>MVEHDKSGSKRQELRSNMRNLITLNKGKFKPTASTAEGDEDDLSFTLLDSVFDTLSDSITCVLGSTDIGAIEVQQFMKDGSRNVLASFNIQTFDDKLLSFVHFADINQLVFVFEQGDIITATYDPVSLDPAETLIEIMGTIDNGIAAAQWSYDEETLAMVTKDRNVVVLSKLFEPISEYHLEVDDLKISKHVTVGWGKKETQFRGKGARAMEREALASLKASGLVGNQLRDPTMPYMVDTGDVTALDSHEITISWRGDCDYFAVSSVEEVPDEDDETKSIKRRAFRVFSREGQLDSASEPVTGMEHQLSWKPQGSLIASIQRKTDLGEEDSVDVIFFERNGLRHGEFDTRLPLDEKVESVCWNSNSEALAVVLANRIQLWTSKNYHWYLKQELYASDISYVKWHPEKDFTLMFSDAGFINIVDFAYKMAQGPTLEPFDNGTSLVVDGRTVNITPLALANVPPPMYYRDFETPGNVLDVACSFSNEIYAAINKDVLIFAAVPSIEEMKKGKHPSIVCEFPKSEFTSEVDSLRQVAFINDSIVGVLLDTDNLSRIALLDIQDITQPTLITIVEVYDKIVLLRSDFDYNHLVYETRDGTVCQLDAEGQLMEITKFPQLVRDFRVKRVHNTSAEDDDNWSAESSELVAFGITNNGKLFANQVLLASAVTSLEITDSFLLFTTAQHNLQFVHLNSTDFKPLPLVEEGVEDERVRAIERGSILVSVIPSKSSVVLQATRGNLETIYPRIMVLAEVRKNIMAKRYKEAFIVCRTHRINLDILHDYAPELFIENLEVFINQIGRVDYLNLFISCLSEDDVTKTKYKETLYSGISKSFGMEPAPLTEMQIYMKKKMFDPKTSKVNKICDAVLNVLLSNPEYKKKYLQTIITAYASQNPQNLSAALKLISELENSEEKDSCVTYLCFLQDVNVVYKSALSLYDVSLALLVAQKSQMDPREYLPFLQELQDNEPLRRKFLIDDYLGNYEKALEHLSEIDKDGNVSEEVIDYVESHDLYKHGLALYRYDSEKQNVIYNIYAKHLSSNQMYTDAAVAYEMLGKLKEAMGAYQSAKRWREAMSIAVQKFPEEVESVAEELISSLTFEHRYVDAADIQLEYLDNVKEAVALYCKAYRYDIASLVAIKAKKDELLEEVVDPGLGEGFGIIAELLADCKGQINSQLRRLRELRAKKEENPYAFYGQETEQADDVSVAPSETSTQESFFTRYTGKTGGTAKTGASRRTAKNKRREERKRARGKKGTIYEEEYLVQSVGRLIERLNQTKPDAVRVVEGLCRRNMREQAHQIQKNFVEVLDLLKANVKEIYSISEKDRERVNENGEVYYIPEIPVPEIHDFPKSHIVDF[2x];> MVECITPEAIFIGANKQTQVSDIHKVKKIVAFGAGKTIALWDPIEPNNKGVYATLKGHEAEVTCVRFVPDSDFMVSASEDHHVKIWKFTDYSHLQCIQTIQHYSKTIVALSALPSLISVGCADGTISIWRQNIQNDEFGLAHEFTIKKGFFYPLCLSLSKVEEKKYLLAIGGTNVNVFIASFILSDSGIEKCRVVAELEGHEDWVKSLAFRHQETPGDYLLCSGSQDRYIRLWRIRINDLIDDSEEDSKKLTLLSNKQYKFQIDDELRVGINFEALIMGHDDWISSLQWHESRLQLLAATADTSLMVWEPDETSGIWVCSLRLGEMSSKGASTATGSSGGFWSCLWFTHERMDFFLTNGKTGSWRMWATKDNIICDQRLGISGATKDVTDIAWSPSGEYLLATSLDQTTRLFAPWIYDASGRKREIATWHEFSRPQIHGYDMICVETVTDTRFVSGGDEKILRSFDLPKGVAGMLQKFVGIQFEEKSEMPDSATVPVLGLSNKAGEDDANEDDEEEEGGNKETPDITDPLSLLECPPMEDQLQRHLLWPEVEKLYGHGFEITCLDISPDQKLIASACRSNNVQNAVIRIFSTENWLEIKPALPFHSLTITRLKFSKDGKFLLSVCRDRKWALWERNMEDNTFELRFKNEKPHTRIIWDADWAPLEFGNVFVTASRDKTVKVWRHQKEPADDYVLEASIKHTKAVTAISIHDSMIREKILISVGLENGEIYLYSYTLGKFELITQLNEDITPADKITRLRWSHLKRNGKLFLGVGSSDLSTRIYSLAYE;> MARHGKGPKTNKKKLAPEKERFIQCCADITLELTDSLTSGTTREINLNGLITKYSKKYKLKQQPRLTDIINSIPDQYKKYLLPKLKAKPVRTASGIAVVAVMCKPHRCPHIAYTGNICVYCPGGPDSDFEYSTQSYTGYEPTSMRAIRARYDPYEQARGRVEQLKQLGHSIDKVEYVLMGGTFMSLPKEYREDFIVKLHNALSGFNGNDIDEAILYSQQSLTKCVGITIETRPDYCTQTHLDDMLKYGCTRLEIGVQSLYEDVARDTNRGHTVRSVCETFAVSKDAGYKVVSHMMPDLPNVGMERDIEQFKEYFENPDFRTDGLKIYPTLVIRGTGLYELWKTGRYKSYSANALVDLVARILALVPPWTRIYRVQRDIPMPLVTSGVDNGNLRELALARMKDLGTTCRDVRTREVGIQEVHHKVQPDQVELIRRDYYANGGWETFLSYEDPKKDILIGLLRLRKASKKYTYRKEFTSQRTSIVRELHVYGSVVPLHSRDPRKFQHQGFGTLLMEEAERIAKEEHGSEKISVISGVGVRNYYGKLGYELDGPYMSKRI;>[2x]MASSSHNPVILLKRILSLTESSPFILCLDSIAQTSYKLIQEFVHQSKSKGNEYPIVYISFETVNKPSYCTQFIDATQMDFVHLVKQIISYLPAATATQAKKHMVIIDSLNYISTEYITRFLSEIASPHCTMVATYHKDIKDENRTVIPDWNNNYPDKLTLLQFMATTIVDIDVVLTGTLDTEEVSELLNEFRIPRGLNNDIFQLRLVNKRKSGRSLEYDFIVNSNTHEYELLSTTKQEEESSSNGLETPEMLQGLTTFNLGTSNKQKLAKDQVALPFLEAQSFGQGGAIVYEYEKDDDYDEEDPYEDPF;>[2x]MGSVQRQDLVLFSDQSVLPAHFFQDSNSHNLFFITHQSCTQPLWMINALVETHVLGSPSSLNESSSSMLPSSTRSHAVLASFIHEQNYFTNSLNKLKIPSNNYNVLDFLSDFIVNNIHNKPRDKILSDVLAKFSAAIQNNPTDTIVIIEQPELLLSLVSGLTCSELNNKFITPLLRQCKVLIIVSNSDIFNIDEYDASVHSSNLQNFYKSSFIKSMINLNLNPLKTGFAKDVTGSLHVCRGGAPIATSNTSLHVVENEYLYLNEKESTKLFYR;>MSFRKRGEILNDRGSGLRGPLLRGPPRTSSTPLRTGNRRAPGNVPLSDTTARLKKLNIADESKTKMGLDSSHVGVRPSPATSQPTTSTGSADLDSILGHMGLPLGNSVLVEEQSTTEFHSILGKLFAAQGIVHNRISDSSADKTRNGDTHVIVLSLNQMFAKELPGIYKGSRKQMKKNLISEEESKVTVQNLNETQRSTPSRYKDLKIAWKYKLADEKRLGSPDRDDIQQNSEYKDYNHQFDITTRLMPAPIASELTFIAPTQPVSTILSQIEQTIKRNDKKLIRIVIPSLLHPAMYPPKMFESSEIIGLMHGVRSLVKKYYERVVLFASISIDIITPPLLVLLRNMFDSVINLEPFNQEMTEFLERVYKSQPGKIQHGLVHILKLPVFTDRGEMRVLKSEWAFKNGRKKFEIEQWGIPVDD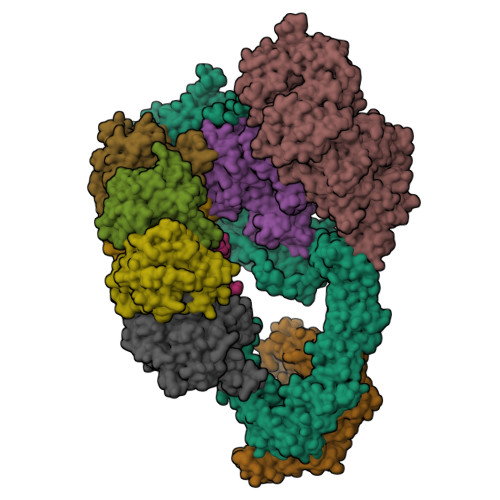AEGSAASEQSHSHSHSDEISHNIPAKKTKISLDY[2x]> MRVKVIDADAFSYIFRTLEEFIDEITLDFTSDGLKIRGIDPSRVTFIDILIPAGYFEEYNVEKEEKVGVKLEDFTDVLKTVTKNDSLYLETDENQNIKVTLDGVYERTFTFPSIVASEIETPNLNLEFPFKAKALTVTFTDIIDEIEDIGGDSIT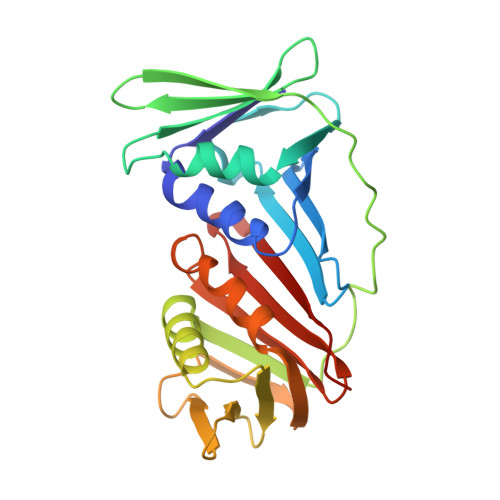FKAEGGKLYLSANSDMGSSTIELSTENGGLLESEGGDAESVYGLEYVVNTSKMRKPSDTVEIAFGSQIPLKLRYNLPQGGYADFYIAPRAE Alanine racemase (Alr) is a pyridoxal-5′-phosphate (PLP)-dependent enzyme that catalyzes the reversible racemization of l- and d-alanine. Since d-alanine is an essential component of the bacterial cell-wall peptidoglycan, and there are no known Alr homologs in humans, this enzyme is being tested as an antibiotic target. Three crystal structures of C. difficile Alr (CdAlr), corresponding to the complex with PLP, the complex with cycloserine and a K271T mutant form of the enzyme with bound PLP, are presented. The structures are prototypical Alr homodimers with two active sites in which the cofactor PLP and cycloserine are localized.

The third structure is that of the K271T mutant enzyme in complex with PLP (CdAlrK271T). To prevent this cleavage, the lysine at position 271 was mutated to a threonine: K271T. Thr was chosen because homologous Alrs from S. aureus, M. tuberculosis, B. anthracis and G. stearothermophilus that are readily purified and crystallized have a Thr at position 271. The structure of CdAlrK271T is the most complete structure and each monomer has ordered main-chain and side-chain electron-density maps for 383 of 385 amino acids with the two disordered residues are at the N-terminus. The topology of CdAlrK271T was chosen to describe the overall enzyme topology since it is the most complete structure. The secondary structure of each monomer is approximately 25% strands, 26% α-helices, 5% 310-helices and 44% loop and turns. CdAlrK271T had a significantly higher catalytic activity than CdAlrWT. Kinetic analyses reveal that the K271T mutant CdAlr has the highest catalytic constants reported to date for any Alr. Lys271 lies on a loop in the substrate entryway of the active site and it has previously been shown that mutations in this region affect the activity of EcAlr. Accordingly, the high catalytic activity of CdAlrK271T could arise from the formation of a tight dimer that hardly dissociates.

>[2x]MQKITVPTWAEINLDNLRFNLNNIKNLLEEDIKICGVIKADAYGHGAVEVAKLLEKEKVDYLAVARTAEGIELRQNGITLPILNLGYTPDEAFEDSIKNKITMTVYSLETAQKINEIAKSLGEKACVHVKIDSGMTRIGFQPNEESVQEIIELNKLEYIDLEGMFTHFATADEVSKEYTYKQANNYKFMSDKLDEAGVKIAIKHVSNSAAIMDCPDLRLNMVRAGIILYGHYPSDDVFKDRLELRPAMKLKSKIGHIKQVEPGVGISYGLTYTTTGKETIATVPIGYADGFTRIQKNPKVLIKGEVFDVVGRICMDQIMVRIDKDIDIKVGDEVILFGEGEVTAERIAKDLGTINYEVLCMISRRVDRVYMENNELVQINSYLLK> MHHHHHHGGSEQKLISEEDLSGGGSWSGSSKEVTERVAELAAEAVRATDKEEVIEIVKELAELAKQSTDSELVNFIVRALAAVAIAAQDKELVIYIVKILAELAKQSTDSELVNEIVKALAEVAKAATDKELVKYIVDILLELAKQADDATLVAKIAEQLAEVREEAKDKELQERIDRVLKKLIEITLRALEESLRE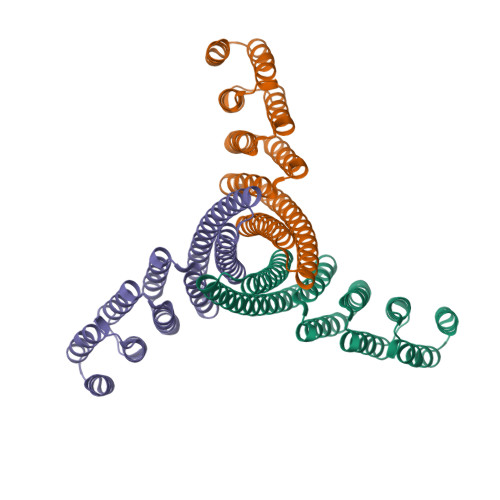LRRILEELKEMLERLEKNPDKDVIVKVLKVIVKAIEASVRNQQISAANQKALALLA> DDKMDYDFKVKLSSERERVEDLFEYEGCKVGRGTYGHVYKAKRKDGKDDKDYALKQIEGTGISMSACREIALLRELKHPNVISLQKVFLSHADRKVWLLFDYAEHDLWHIIKFHRASKANKKPVQLPRGMVKSLLYQILDGIHYLHANWVLHRDLKPANILVMGEGPERGRVKIADMGFARLFNSPLKPLADLDPVVVTFWYRAPELLLGARHYTKAIDIWAIGCIFAELLTSEPIFHCRQEDIKTSNPYHHDQLDRIFNVMGFPADKDWEDIKKMPEHSTLMKDFRRNTYTNCSLIKYMEKHKVKPDSKAFHLLQKLLTMDPIKRITSEQAMQDPYFLEDPLPTSDVFAGCQIPYPKREFLTEEEPDDKGDKKNQQQQQGNNHTNGTGHPGNQDSSHTQGPPLKK;> DKAMAGNFWQSSHYLQWILDKQDLLKERQKDLKFLSEEEYWKLQIFFTNVIQALGEHLKLRQQVIATATVYFKRFYARYSLKSIDPVLMAPTCVFLASKVEEFGVVSNTRLIAAATSVLKTRFSYAFPKEFPYRMNHILECEFYLLELMDCCLIVYHPYRPLLQYVQDMGQEDMLLPLAWRIVNDTYRTDLCLLYPPFMIALACLHVACVVQQKDARQWFAELSVDMEKILEIIRVILKLYEQWKNFDERKE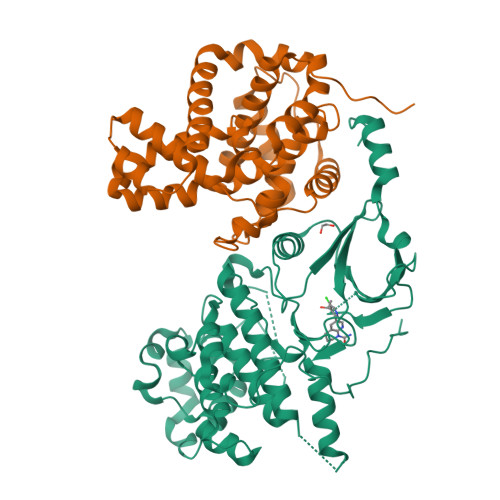MATILSKMPKPKPPPNSEGEQGPNGSQNSSY>[8x]GSSHHHHHHSSGLVPGGSHMVSKGEENNMAVIKPDMKIKLRMEGAVNGHPFAIEGVGLGKPFEGKQSMDLKVKEGGPLPFAYDILTTVFXNRVFAKYPENIVDYFKQSFPEGYSWERSMNYEDGGICNATNDITLDGDCYIYEIRFDGVNFPANGPVMQKRTVKWEPSTEKLYVRDGVLKGDVNTALSLEGGGH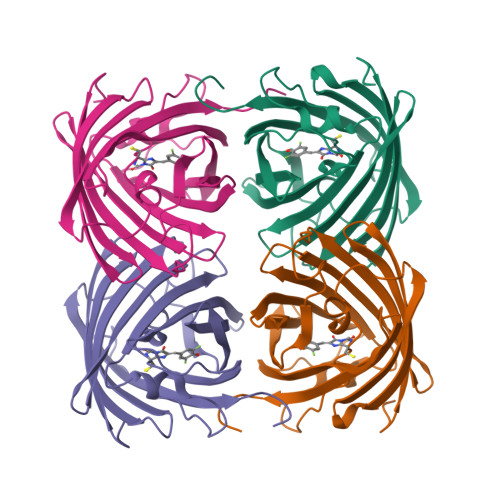YRCDFKTTYKAKKVVQLPDYHFVDHHIEIKSHDKDYSNVNLHEHAEAHSGLPRQAMDELYK> QPVLHLVALNTPLSGGMRGIRGADFQCFQQARAVGLSGTFRAFLSSRLQDLYSIVRRADRGSVPIVNLKDEVLSPSWDSLFSGSQGQLQPGARIFSFDGRDVLRH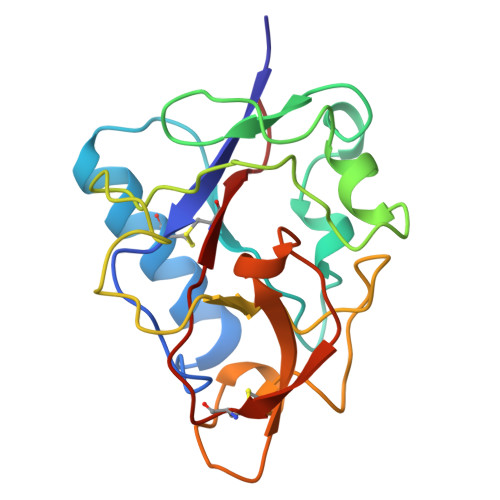PAWPQKSVWHGSDPSGRRLMESYCETWRTETTGATGQASSLLSGRLLEQKAASCHNSYIVLCIENSF> GHMAKQYDSVECPFCD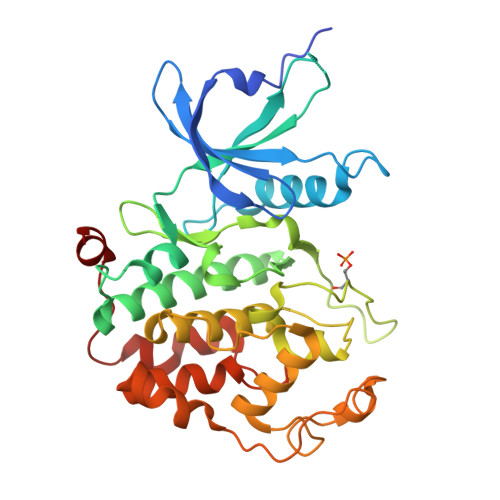EVSKYEKLAKIGQGTFGEVFKARHRKTGQKVALKKVLMENEKEGFPITALREIKILQLLKHENVVNLIEICRTKASPYNRCKGSIYLVFDFCEHDLAGLLSNVLVKFTLSEIKRVMQMLLNGLYYIHRNKILHRDMKAANVLITRDGVLKLADFGLARAFSLAKNSQPNRYTNRVVTLWYRPPELLLGERDYGPPIDLWGAGCIMAEMWTRSPIMQGNTEQHQLALISQLCGSITPEVWPNVDNYELYEKLELVKGQKRKVKDRLKAYVRDPYALDLIDKLLVLDPAQRIDSDDALNHDFFWSDPMPSDLKGMLST> GPGSGDPYWAYSGAYGPEHWVTSSVSCGGSHQSPIDILDHHARVGDEYQELQLDGFDNESSNKTWMKNTGKTVAILLKDDYFVSGAGLPGRFKAEKVEFHWGHSNGSAGSEHSVNGRRFPVEMQIFFYNPDDFDSFQTAISENRIIGAMAIFFQVSPRDNSALDPIIHGLKGVVHHEKETFLDPFILRDLLPASLGSYYRYTGSLTTPPCSEIVEWIVFRRPVPISYHQLEAFYSIFTTEQQDHVKSVEYLRNNFRPQQALNDRVV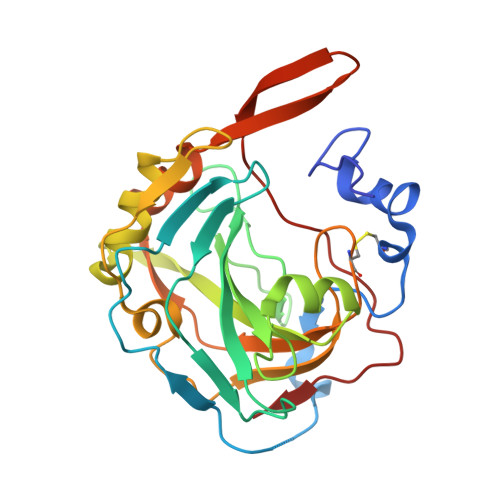SKS>MKERLEKLVKFMDENSIDRVFIAKPVNVYYFSGTSPLGGGYIIVDGDEATLYVPELEYEMAKEESKLPVVKFKKFDEIYEILKNTETLGIEGTLSYSMVENFKEKSNVKEFKKIDDVIKDLRIIKTKEEIEIIEKACEIADKAVMAAIEEITEGKREREVAAKVEYLMKMNGAEKPAFDTIIASGHRSALPHGVASDKRIERGDLVVIDLGALYNHYNSDITRTIVVGSPNEKQREIYEIVLEAQKRA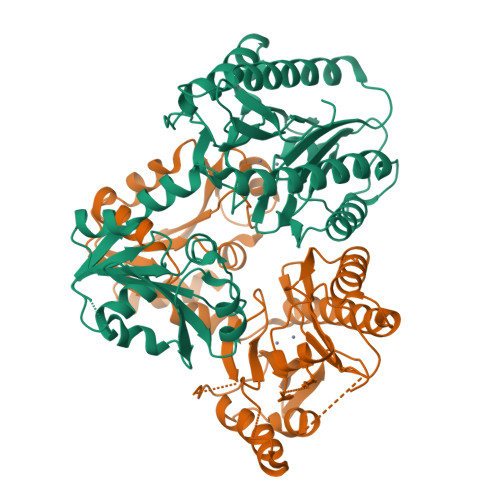VEAAKPGMTAKELDSIAREIIKEYGYGDYFIHSLGHGVGLEIHEWPRISQYDETVLKEGMVITIEPGIYIPKLGGVRIEDTVLITENGAKRLTKTERELL[2x]During HIV infection, specific RNA-protein interaction between the Rev response element (RRE) and viral Rev protein is required for nuclear export of intron-containing viral mRNA transcripts. Rev initially binds the high-affinity site in stem-loop II, which promotes oligomerization of additional Rev proteins on RRE. Two Rev-binding sites have been identified within RRE, a high-affinity site within stem-loop II (SLII) and a secondary binding site within stem I. SLII forms a three-stem structure, IIA-C, and a purine-rich internal loop within stem IIB is predicted to be the initial high-affinity Rev-binding site. Rev oligomerization is required for the biological activity of the Rev–RRE complex, as binding of a single Rev molecule is insufficient for nuclear export.

The crystal structure of RRE SLII was determined using the tRNA-scaffold approach, where the 67 nt of HIV-1 RRE SLII replaced the anticodon loop of the human tRNALys (134 nt total). To facilitate crystallization, a guanine nucleotide (G23) was added to the apical loop of stem IIB to form a tetraloop structure (5′-AAUG-3′). The RNA crystallized in space group P21 with two molecules in the asymmetric unit, and the structure was determined to 2.85 Å resolution. The two RRE SLII molecules in the crystallographic asymmetric unit adopted two different conformations, one “closed” and the other “open”. Both molecules are “lambda (λ)”-shaped and consist of stems IIA, IIB, and IIC connected by a three-way junction. Stem IIB is coaxially stacked on stem IIA, and stem IIC projects out from the three-way junction at a ~70° angle to stem IIA. Our RRE SLII structure now shows that the purine-rich, high-affinity Rev-binding site (the GGG motif) is incorporated into the three-way junction rather than the predicted internal loop in stem IIB. The closed and open conformers differ in non-canonical base pair interactions within the initial high-affinity Rev-binding site (8GGGCG12/32CGGUACA38). In the closed conformation, the A-form helical structure is maintained at the triple guanine motif (8GGG10) via non-canonical base-pairing interactions of G8·U35 and G9·G34. The open conformation is marked by a non-canonical purine–purine base pair between G10 and G34 and melting of the G8·U35 base pair interactions at the base of stem IIB.

>GCCCGGAUAGCUCAGUCGGUAGAGCAGCGGGCACUAUGGGCGCAGUGUCAAUGGACGCUGACGGUACAGGCCAGACAAUUAUUGUCUGGUAUAGUGCCCGCGGGUCCAGGGUUCAAGUCCCUGUUCGGGCGCCA[2x]2-DEOXY-GLUCITOL-6-PHOSPHATE 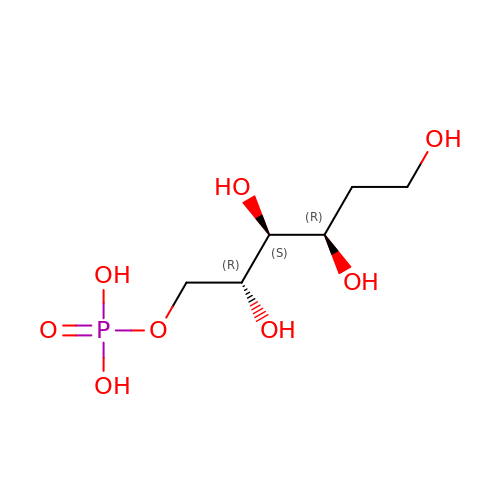| C6 H15 O8 P | KLPBNGZTTQNYHR-PBXRRBTRSA-N> MNETGSIGIIETKYAEFKELILNNGSVLSPVVIAYET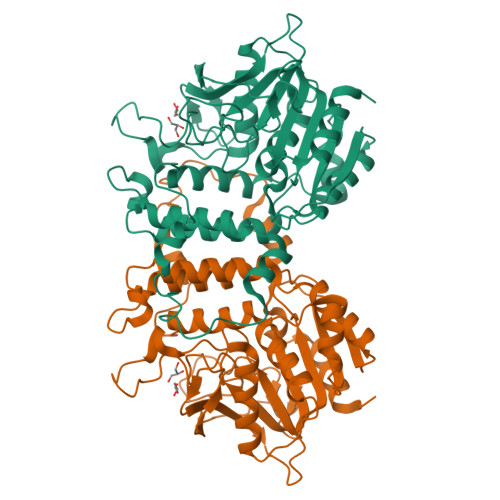YGTLSSSKNNAILICHALSGDAHAAGYHSGSDKKPGWWDDYIGPGKSFDTNQYFIICSNVIGGCKGSSGPLSIHPETSTPYGSRFPFVSIQDMVKAQKLLVESLGIEKLFCVAGGSMGGMQALEWSIAYPNSLSNCIVMASTAEHSAMQIAFNEVGRQAILSDPNWKNGLYDENSPRKGLALARMVGHITYLSDDKMREKFGRNPPRGNILSTDFAVGSYLIYQGESFVDRFDANSYIYVTKALDHYSLGKGKELTAALSNATCRFLVVSYSSDWLYPPAQSREIVKSLEAADKRVFYVELQSGEGHDSFLLKNPKQIEILKGFLENPN>SFMVSLESSRTQYVNQLRSHAQDAATALALSLTPNIDDPAMVELLVSSIFDSGYYSSIRVVDLKTDQTIVERNGIPAVTNVPDWFVKLIGLEPAGGDALVSRGWEQAARVEVVSHPMFALAKLWQSALGS[2x]

Here, we elucidated the molecular mechanism underlying the function and regulation of P. fluorescens LapD, a transmembrane receptor essential for biofilm formation in this strain. As c-di-GMP levels change LapD switches between two states: the dinucleotide-unbound off state that retards stable biofilm formation by facilitating the secretion of the cell surface adhesin LapA, and the c-di-GMP-bound on state that supports cell adhesion by preventing the release of LapA from the outer membrane. Binding of c-di-GMP to the LapD EAL domain is relayed to the periplasmic output domain through an inside-out signaling mechanism that utilizes a juxtamembrane HAMP domain, a relay module often found in bacterial transmembrane receptors. Here, we present three crystal structures of LapD from P. fluorescens that provide models for the c-di-GMP-unbound cytoplasmic domain lacking only the HAMP domain, a c-di-GMP-bound EAL domain dimer, and the periplasmic domain.

In order to shed light on how changes in the cytosolic domain are sensed in the periplasm, we determined the structure of the entire output domain (residues 22–151). Crystals grown with selenomethionine-derivatized protein diffracted X-rays to a maximum resolution of 1.8 Å. The structure was solved by single-wavelength anomalous dispersion phasing. The final model consists of two molecules per asymmetric unit spanning residues 23–150. The periplasmic output domain of LapD forms an extensively interwoven, domain-swapped dimer sharing 3,429 Å2 interfacial surface area between the protomers (1/3 of LapD's output domain molecular surface). The dimer adopts an overall V-shaped conformation. Each arm of the fold consists of two α-helices and two β-strands contributed by one of the two protomers, complemented by two β-strands flanked by helical segments from the other. The two half sites are linked via a long connecting segment that crosses over at the center of the dimer. The other striking feature is a strictly conserved loop connecting the strands β3 and β4 formed by the conserved GWxQ motif (residues 124–127 of LapD). W125 forms the most distal point of the periplasmic domain located at the center of the loop, and its side chain is in an outward-facing rotamer conformation.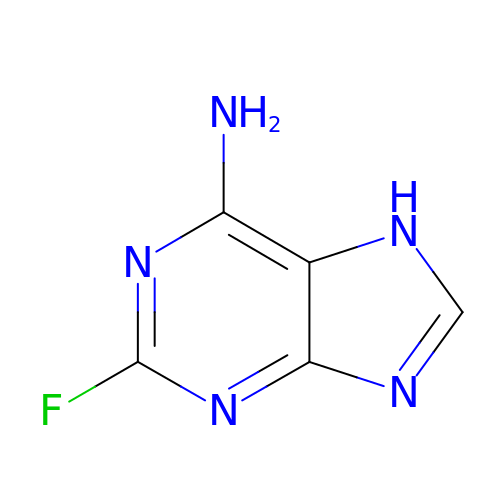2-fluoroadenine | C5 H4 F N5 | WKMPTBDYDNUJLF-UHFFFAOYSA-N>[4x]MLEIKRYKNRVASRKSRAKFKQLLQHYREVAAAKSSENDRLRLLLKQMCPSLDVDSIIPRTPD

The viral bZIP transcription factor ZEBRA (Zta, BZLF1) regulates this cycle by binding to two classes of ZEBRA response elements (ZREs): CpG-free motifs resembling the consensus AP-1 site recognized by cellular bZIP proteins and CpG-containing motifs that are selectively bound by ZEBRA upon cytosine methylation. ZEBRA is a homodimeric protein related to the activating protein 1 (AP-1) family of bZIP transcription factors. ZEBRA regulates the EBV infection cycle by playing key roles both in establishing viral latency and triggering lytic replication. Underpinning ZEBRA’s dual role in prelatency and lytic activation is its ability to recognize two distinct classes of DNA target sites, collectively termed ZEBRA responsive elements (ZREs).

We crystallized ZEBRA’s DNA-binding domain in complex with a 19 base-pair (bp) DNA duplex containing the CpG-methylated ZRE2 site in the EBV promoter Rp (TGAGmCGA; hereafter meZRE2) and solved the structure at 2.5 Å resolution by molecular replacement. Unlike the single helix of a canonical bZIP domain, whose N- and C-terminal residues bind DNA and mediate coiled-coil dimer formation, respectively, ZEBRA’s C-terminal region folds back on and stabilizes an unusually short coiled coil. Our crystal structure closely resembles previous ZEBRA structures bound to the AP-1 site and to the Rp meZRE2 site in an alternate crystal form, apart from the dimerization domain which exhibits variable bending. Each ZEBRA monomer recognizes one of the two meZRE2 half-sites, which we denote ‘A’ (half-site shared with AP-1) and ‘M’ (methylated half-site). Consequently, only a single (hereafter ‘CpG-proximal’) monomer senses the methylation state of meZRE2. The CpG-proximal monomer recognizes DNA bases in the M half-site through direct H-bonding interactions of Asn182 with G2, Ser186 with mC–2′ and mC1, and Arg190 with G0 and G–1′, while electrostatic interactions with the DNA backbone resemble those in the A half-site. Strikingly, the Ser186 side chain is positioned precisely on the local dyad axis that relates the two CpG methylation marks, allowing it to hydrogen bond with both mC bases. By contrast, in the methylated complex the mC1 methyl group sterically selects for the g+ rotamer, thereby stabilizing the H-bonds with the mC bases. In the AP-1 complex, the Arg190 guanidino group forms bidentate H-bonds and is coplanar with the G0 base, whereas in the meZRE2 complex it twists out of this plane to form a bifurcated H-bond with the G–1′ base on the opposite strand. The resulting configuration is strikingly similar to the mC-Arg-G triad observed in methyl-CpG binding proteins (MBPs), whereby a conserved arginine hydrogen bonds with the G base of the CpG motif and contacts the methyl group of the adjacent mC base (analogous to G–1′ and mC–2′ in our structure).> SSKNEWRKSAIANTLLYLRLKNIYVSADDFVEEQNVYVLPKNLLKKFIEISDVKIQVAAFIYGMSAKDHPKVKEIKTVVLVPQLGHVGSVQISNIPDIGDLPDTEGLELLGWIHTQTEELKFMAASEVATHSKLFADKKRDCIDISIFSTPGSVSLSAYNLTDEGYQWGEENKDIMNVLSEGFEPTFSTHAQLLLSDRITGNFIIPSGNVWNYTFMGTAFNQEGDYNFKYGIPLEFYNEMHRPVHFLQFSELAGDEELEAEQIDVFS;> MTEHETKDKAKKIREIYRYDEMSNKVLKVDKRFMNTSQNPQRDAEISQPKSMSGRISAKDMGQGLCNNINKGLKENDVAVEKTGKSASLKKIQQHNTILNSSSDFRLHYYPKDPSNVETYEQILQWVTEVLGNDIPHDLIIGTADIFIRQLKENEENEDGNIEERKEKIQHELGINIDSLKFNELVKLMKNITDYETHPDNSNKQAVAILADDEKSDEEEVTEMSNNANVLGGEINDNEDDDEEYDYNDVEVNSKKKNKRA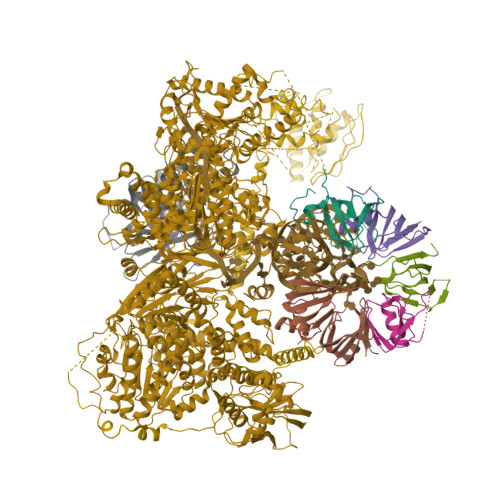LPNIENDIIKLSDSKTSNIESVPIYSIDEFFLQRKLRSELGYKDTSVIQDLSEKILNDIETLEHNPVALEQKLVDLLKFENISLAEFILKNRSTIFWGIRLAKSTENEIPNLIEKMVAKGLNDLVEQYKFRETTHSKRELDSGDDQPQSSEAKRTKFSNPAIPPVIDLEKIKFDESSKLMTVTKVSLPEGSFKRVKPQYDEIHIPAPSKPVIDYELKEITSLPDWCQEAFPSSETTSLNPIQSKVFHAAFEGDSNMLICAPTGSGKTNIALLTVLKALSHHYNPKTKKLNLSAFKIVYIAPLKALVQEQVREFQRRLAFLGIKVAELTGDSRLSRKQIDETQVLVSTPEKWDITTRNSNNLAIVELVRLLIIDEIHLLHDDRGPVLESIVARTFWASKYGQEYPRIIGLSATLPNYEDVGRFLRVPKEGLFYFDSSFRPCPLSQQFCGIKERNSLKKLKAMNDACYEKVLESINEGNQIIVFVHSRKETSRTATWLKNKFAEENITHKLTKNDAGSKQILKTEAANVLDPSLRKLIESGIGTHHAGLTRSDRSLSEDLFADGLLQVLVCTATLAWGVNLPAHTVIIKGTDVYSPEKGSWEQLSPQDVLQMLGRAGRPRYDTFGEGIIITDQSNVQYYLSVLNQQLPIESQFVSKLVDNLNAEVVAGNIKCRNDAVNWLAYTYLYVRMLASPMLYKVPDISSDGQLKKFRESLVHSALCILKEQELVLYDAENDVIEATDLGNIASSFYINHASMDVYNRELDEHTTQIDLFRIFSMSEEFKYVSVRYEEKRELKQLLEKAPIPIREDIDDPLAKVNVLLQSYFSQLKFEGFALNSDIVFIHQNAGRLLRAMFEICLKRGWGHPTRMLLNLCKSATTKMWPTNCPLRQFKTCPVEVIKRLEASTVPWGDYLQLETPAEVGRAIRSEKYGKQVYDLLKRFPKMSVTCNAQPITRSVMRFNIEIIADWIWDMNVHGSLEPFLLMLEDTDGDSILYYDVLFITPDIVGHEFTLSFTYELKQHNQNNLPPNFFLTLISENWWHSEFEIPVSFNGFKLPKKFPPPTPLLENISISTSELGNDDFSEVFEFKTFNKIQSQVFESLYNSNDSVFVGSGKGTGKTAMAELALLNHWRQNKGRAVYINPSGEKIDFLLSDWNKRFSHLAGGKIINKLGNDPSLNLKLLAKSHVLLATPVQFELLSRRWRQRKNIQSLELMIYDDAHEISQGVYGAVYETLISRMIFIATQLEKKIRFVCLSNCLANARDFGEWAGMTKSNIYNFSPSERIEPLEINIQSFKDVEHISFNFSMLQMAFEASAAAAGNRNSSSVFLPSRKDCMEVASAFMKFSKAIEWDMLNVEEEQIVPYIEKLTDGHLRAPLKHGVGILYKGMASNDERIVKRLYEYGAVSVLLISKDCSAFACKTDEVIILGTNLYDGAEHKYMPYTINELLEMVGLASGNDSMAGKVLILTSHNMKAYYKKFLIEPLPTESYLQYIIHDTLNNEIANSIIQSKQDCVDWFTYSYFYRRIHVNPSYYGVRDTSPHGISVFLSNLVETCLNDLVESSFIEIDDTEAEVTAEVNGGDDEATEIISTLSNGLIASHYGVSFFTIQSFVSSLSNTSTLKNMLYVLSTAVEFESVPLRKGDRALLVKLSKRLPLRFPEHTSSGSVSFKVFLLLQAYFSRLELPVDFQNDLKDILEKVVPLINVVVDILSANGYLNATTAMDLAQMLIQGVWDVDNPLRQIPHFNNKILEKCKEINVETVYDIMALEDEERDEILTLTDSQLAQVAAFVNNYPNVELTYSLNNSDSLISGVKQKITIQLTRDVEPENLQVTSEKYPFDKLESWWLVLGEVSKKELYAIKKVTLNKETQQYELEFDTPTSGKHNLTIWCVCDSYLDADKELSFEINVK;> AAAAAAAAAAAAAAAAAAAAAAAAAAAAAAAAAAAAAAAAAAAAAAAAAAAAAAAAAAAAAAAAAAAAAAAAAAAAAAAAAAAAAAAAAAAAAAAAAAAAAAAAAAAAAAAAAAAAAAAAAAAAAAAAAAAAAAAAAAAAAAAAAAAAAAAAAAAAAAAAAAAAAAAAAAAAAAAAAAAAAAAAAAAAAAAAAAAAAAAAAAAAAAAAAAAAAAAAAAAAAAAAAAAAAAAAAAAAAAAAAAAAAAAAAAAAAAAAAAAAAAAAAAAAARAAAAAAAAAAAAAAAAAAAAAAAAAAAAAAAAAAAAAAAAAAAAAAATTKEAYKKLSQKFHGTKSNKK;> MSKIQVAHSSRLANLIDYKLRVLTQDGRVYIGQLMAFDKHMNLVLNECIEERVPKTQLDKLRPRKDSKDGTTLNIKVEKRVLGLTILRGEQILSTVVEDKPLLSKKERLVRDKKEKKQAQKQTKLRKEKEKKPGKIAKPNTANAKHTSSNSREIAQPSSSRYNGGNDNIGANRSRFNNEAPPQTRKFQPPPGFKRK;> MKLVNFLKKLRNEQVTIELKNGTTVWGTLQSVSPQMNAILTDVKLTLPQPRLNKLNSNGIAMASLYLTGGQQPTASDNIASLQYINIRGNTIRQIILPDSLNLDSLLVDQKQLNSLRRSGQIANDPSKKRRRDFGAPANKRPRRGL;> MSSQIIDRPKHELSRAELEELEEFEFKHGPMSLINDAMVTRTPVIISLRNNHKIIARVKAFDRHCNMVLENVKELWTEKKGKNVINRERFISKLFLRGDSVIVVLKTPVE;> MTMNGIPVKLLNEAQGHIVSLELTTGATYRGKLVESEDSMNVQLRDVIATEPQGAVTHMDQIFVRGSQIKFIVVPDLLKNAPLFKKNSSRPMPPIRGPKRR;> MSNKVKTKAMVPPINCIFNFLQQQTPVTIWLFEQIGIRIKGKIVGFDEFMNVVIDEAVEIPVNSADGKEDVEKGTPLGKILLKGDNITLITSAD;> MSESSDISAMQPVNPKPFLKGLVNHRVGVKLKFNSTEYRGTLVSTDNYFNLQLNEAEEFVAGVSHGTLGEIFIRCNNVLYIRELPN;> MVSTPELKKYMDKKILLNINGSRKVAGILRGYDIFLNVVLDDAMEINGEDPANNHQLGLQTVIRGNSIISLEALDAI>KHSLPDLPYDYGALEPHINAQIMQLHHSKHHAAYVNNLNVTEEKYQEALAKGDVTAQIALQPALKFNGGGHINHSIFWTNLSPNGGGEPKGELLEAIKRDFGSFDKFKEKLTAASVGVQGSGWGWLGFNKERGHLQIAACPNQ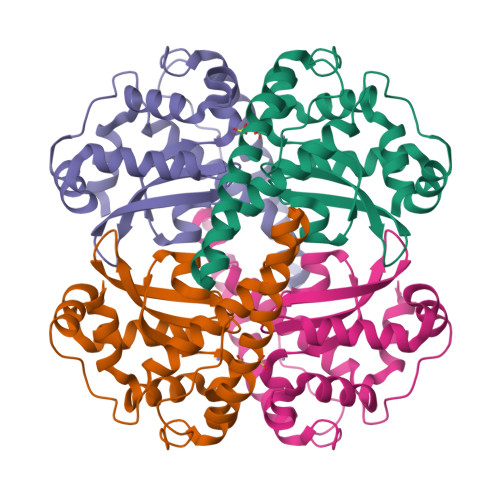DPLQGTTGLIPLLGIDVWAHAYYLQYKNVRPDYLKAIWNVINWENVTERYMACKK[2x]> SHMAVIRIADERDRVQKKTFTKWVNKHLIKHWRAEAQRHISDLYEDLRDGHNLISLLEVLSGDSLPREKGR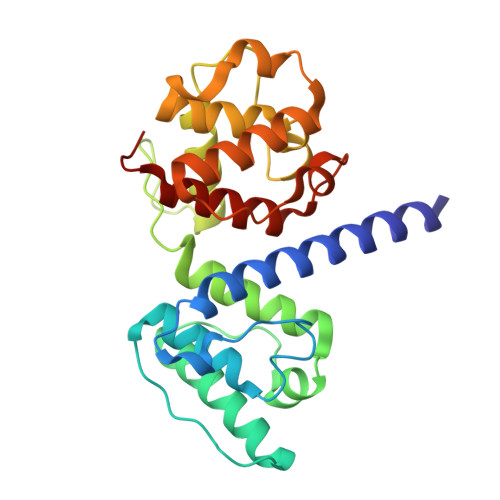MRFHKLQNVQIALDYLRHRQVKLVNIRNDDIADGNPKLTLGLIWTIILHFQISDIQVSGQSEDMTAKEKLLLWSQRMVEGYQGLRCDNFTSSWRDGRLFNAIIHRHKPLLIDMNKVYRQTNLENLDQAFSVAERDLGVTRLLDPEDVDVPQPDEKSIITYVSSLYDAMPRVP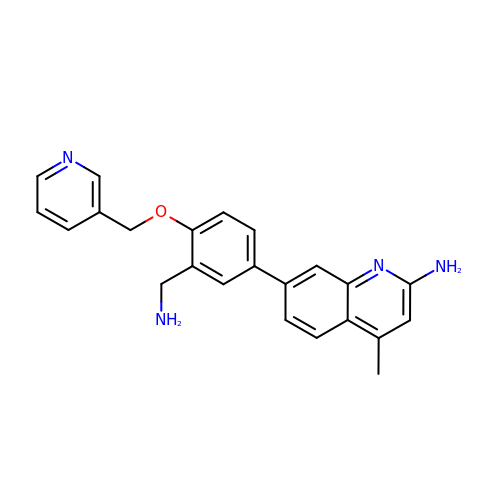7-{3-(aminomethyl)-4-[(pyridin-3-yl)methoxy]phenyl}-4-methylquinolin-2-amine | C23 H22 N4 O | RSZQDXJFSPTWRD-UHFFFAOYSA-N>[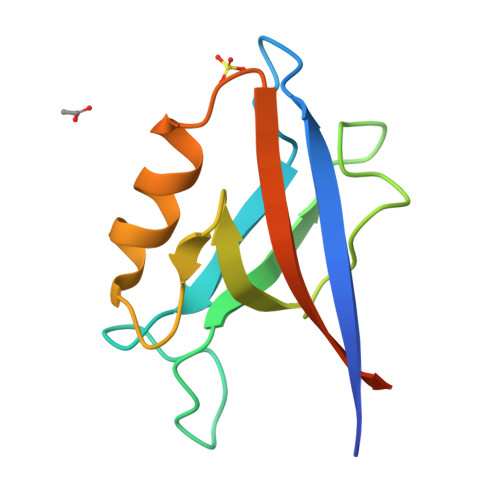3x]GSHMIWEQHTVTLHRAPGFGFGIAISGGRDNPHFQSGETSIVISDVLKGGPAEGQLQENDRVAMVNGVSMDNVEHAFAVQQLRKSGKNAKITIRRKKGGGESLTGYV>[4x]SGISLDNSYKMDYPEMGLCIIINNKNFHKSTGMTSRSGTDVDAANLRETFRNLKYEVRNKNDLTREEIVELM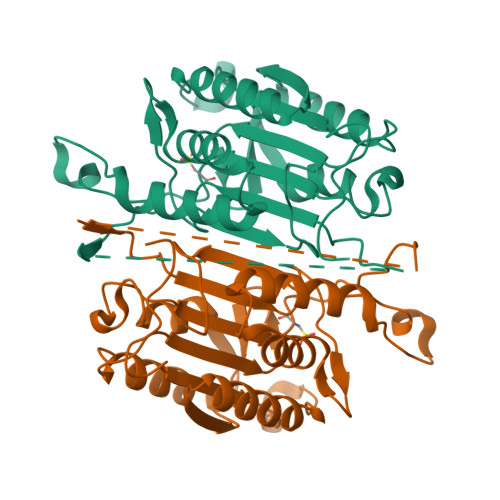RDVSKEDHSKRSSFVCVLLSHGEEGIIFGTNGPVDLKKITNFFRGDRCRSLTGKPKLFIIQACRGTELDCGIETDSGVDDDMACHKIPVDADFLYAYSTAPGYYSWRNSKDGSWFIQSLCAMLKQYADKLEFMHILTRVNRKVATEFESFSFDATFHAKKQIPCIVSMLTKELYFYH> SYVMPQPTSQQRASVASSQSTQGAVGWSAATGWVVLFVAVALVVWFVSLDMRHLVGPDEGRYAEISREMFASGDWVTIRYNALKYFEKPPFHMWVTVVGYELFGLGEWQARLAVALSGLLGIGVSMMAARRWFGARAAAFTGLALLAAPMWSVAAHFNTLDMTLAGVMSCVLAFMLMGQHPDASVAARRGWMVACWAAMGVAILTKGLVGIALPGLVLVVYTLVTRDWGLWRRLHLALGVVVMLVITVPWFYLVSVRNPEFPNFFFIHEHWQRYTSNIHSRSGSVFYFLPLVIGGFLPWAGIFPKLWTAMRAPVEGTQARFRPALMAGIWAIAIFVFFSISR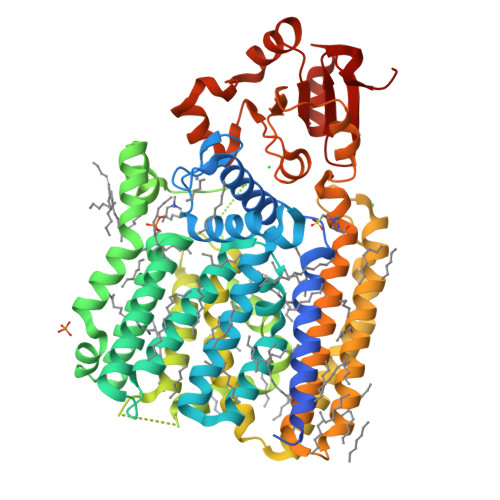SKLPGYIVPVIPALGILAGVALDRLSPRSWGKQLIGMAIVAACGLLASPVVATLNANHIPNSFYRAYAVWVAVAFVVMLLGIAVARLLLRRGVLPSVAVYAMGMYLGFTVALLGHETVGRPASGADIAPQIAQKLTPEMPLYGVQMLDHTLPFYLRHPLMMVGQADELTFGATVEPQRVVPDVDSFTKLWKNGQPAMAVMSPDTYLALAPTLSMYVVARDWRRVVVANVASLAGPQ>MGITLGEVFPNFEADSTIGKLKFHDWLGNSWGVLFSHPRDFTPVSTTELGRVIQLEGDFKKRGVKLIALSCDNVADHKEWSEDVKCLSGVKGDMPYPIIADETRELAVKLGMVDPDERTSTGMPLTCRAVFIIGPDKKLKLSILYPATTGRNFSEILRVIDSLQLTAQKKVATPADWQPGDRCMVVPGVSAEEA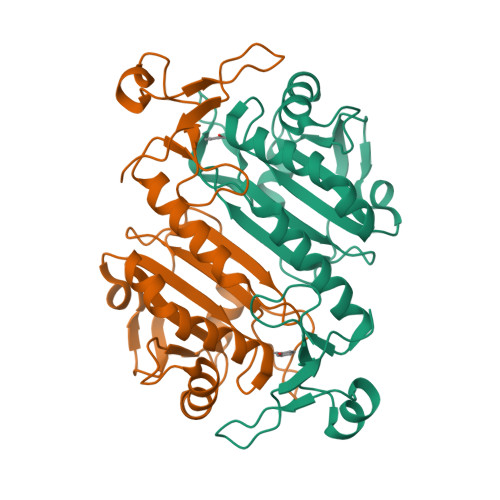KTLFPNMEVKAVPSGKGYLRYTPQPKSMGGSRSHHHHHH[8x]> MSLSSGRTVPTRSHGLGKEGVSTTGASQVEFGDPELTARINDAMVQVEELLHTELSSGEDFLVDIVMHLTRAGGKRFRPMFALLASEFGEKPLSENVIKAAVVVEITHLATLYHDDVMDEASMRRGVPSANARWDNSVAILAGDILLAHASGLMSQLGTDTVAHFAETFGELVTGQMRETVGPRDTDPIEHYTNVIREKTGVLIASAGYLGAMHAGAAPEHIDALKNFGAAVGMIFQIVDDIIDIFSETHESGKTPGTDLREGVFTLPVLYALREDTPVGAELRDILTGPLEDDETVNHVLELLSQSGGRQAAL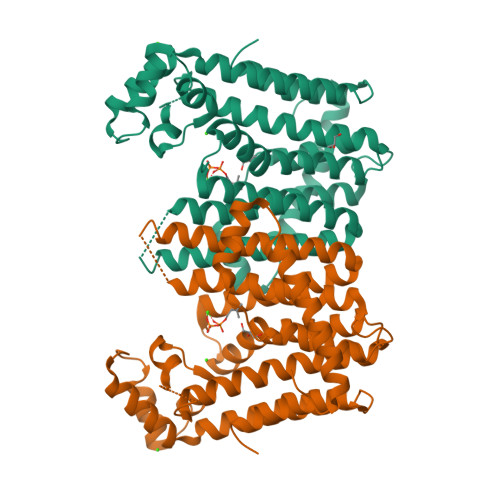DEVYRYMDIANAELDRLPDSTVKEALRNLATFTVKRVGEGHHHHHH1-METHYLQUINOLIN-2(1H)-ONE | C10 H9 N O | 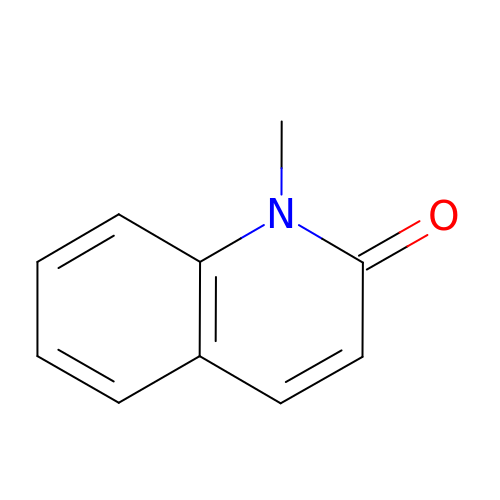QYEMNJMSULGQRD-UHFFFAOYSA-N> MLRRSDLLLKKGWTHNPGRTRRGGKNLAWRPKMSERTLEQFVPLHLAFPRRHPNSWQERQFHLLGYVKWPKEIGFYNAGDNFELTPQAAYRIYKQNCDETFWTRLHNEKTI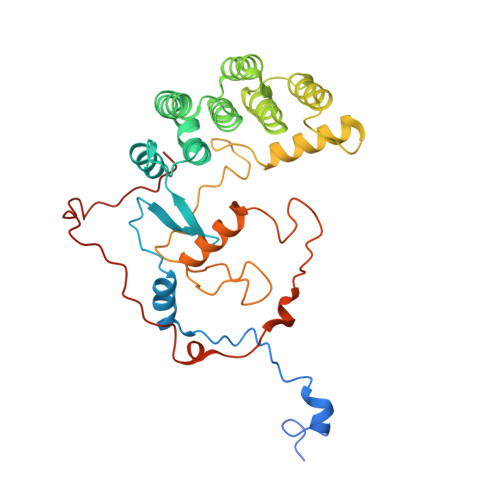IHLLPLVEQDPGTNMVLVDDIFRHHLKRFGADHYIYNAVMQAAAFAKDFPRCEQLLAEMRGLGLEPNAQSYVNMMLGARLTGKPRDQAEAFFREGIKTGAISAVMRLDTEFQMWMNQLERLGSFKAKVGYLSVNEEGASPMPRDMWALWGWHRTEAKFISRKQMISEQVQNRVRSGKELVGTVYQKARRQPWAKYNGMFPYDYNGPARRPAASFVDAPTPTHNAEVCGTAYA>[8x]MLRAAARFGPRLGRRLLSAAATQAVPAPNQQPEVFCNQIFINNEWHDAVSRKTFPTVNPSTGEVICQVAEGDKEDVDKAVKAARAAFQLGSPWRRMDASHRGRLLNRLADLIERDRTYLAALETLDNGKPYVISYLVDLDMVLKCLRYYAGWADKYHGKTIPIDGDFFSYTRHEPVGVCGQIIPWNFPLLMQAWKLGPAL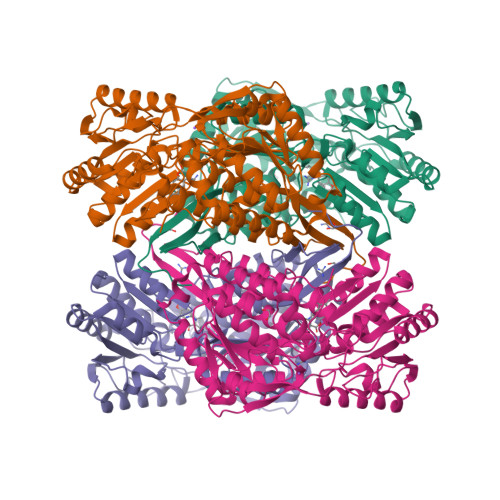ATGNVVVMKVAEQTPLTALYVANLIKEAGFPPGVVNIVPGFGPTAGAAIASHEDVDKVAFTGSTEIGRVIQVAAGSSNLKRVTLELGGKSPNIIMSDADMDWAVEQAHFALFFNQGQCCCAGSRTFVQEDIYDEFVERSVARAKSRVVGNPFDSKTEQGPQVDETQFKKILGYINTGKQEGAKLLCGGGIAADRGYFIQPTVFGDVQDGMTIAKEEIFGPVMQILKFKTIEEVVGRANNSTYGLAAAVFTKDLDKANYLSQALQAGTVWVNCYDVFGAQSPFGGYKMSGSGRELGEYGLQAYTEVKTVTVKVPQKNS>AQPDIKFASKEYGVTIGESRIIYPLDAAGVMVSVKNTQDYPVLIQSRIYDENKEKESEDPFVVTPPLFRLDAKQQNSLRIAQAGGVFPRDKESLKWLCVKGIPPKDEDIWVDDATNKQKFNPDKDVGVFVQFAINNCIKLLVRPNELKGTPIQFAENLSWKVDGGKLIAENPSPFYMN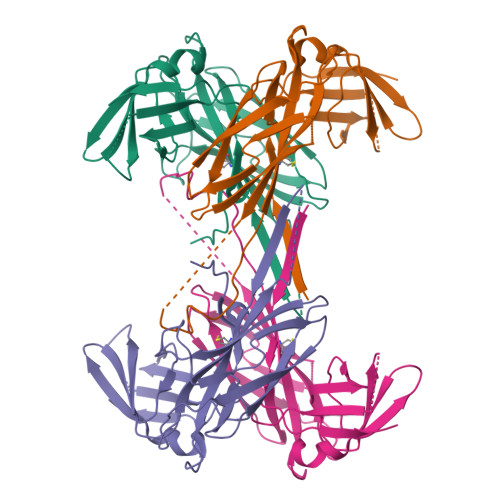IGELTFGGKSIPSHYIPPKSTWAFDLPKGLAGARNVSWRIINDQGGLDRLYSKNVTL[6x]> MDRPEGSEERTVQTSNVVLGETNIESQDIASKEYSPTWDRLASSEVSDEYPMLTDRWLFWKSVKWEVN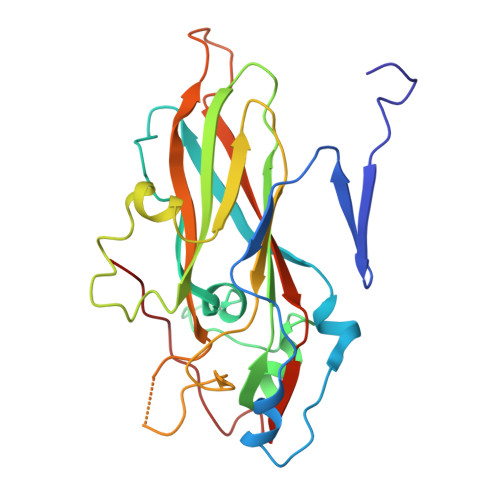DSAFGKMLVQEKFPQSWVQMDVNVNNIPRYTNIPNFIPFNIHQYMRADFEVKIYVNPNDFVSGWLIMAFLYQGSEMFDYKLRRNPAALMQMPHVLVNVGAANEATLKIPYRYVRPFMRCKDILRGDNLITGVTEPLNMGVLFVEVLIPFRTSAASSAPKSLDVSLFVKMTNAKFTGMVDGSIALLSKPIALPE>[2x]SGSFELSVQDLNDLLSDGSGCYSLPSQPCNEVTPRIYVGNASVAQDIPKLQKLGITHVLNAAEGRSFMHVNTNANFYK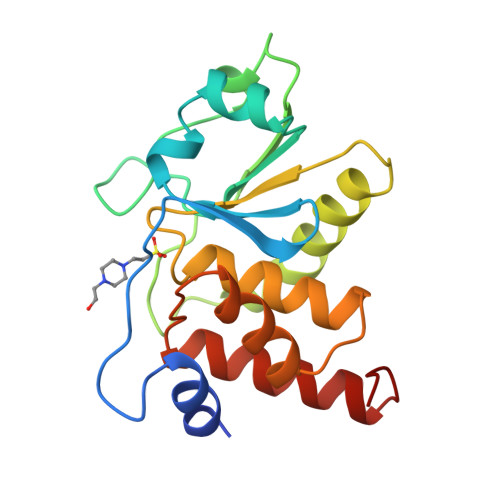DSGITYLGIKANDTQEFNLSAYFERAADFIDQALAQKNGRVLVHCREGYSRSPTLVIAYLMMRQKMDVKSALSIVRQNREIGPNDGFLAQLCQLNDRLAKEGKLKP> GVALGATRVIYPAGQKQEQLAVTNNDENSTYLIQSWVENADGVKDGRFIVTPPLFAMKGKKENTLRILDATNNQLPQDRESLFWMNVKAIPSMDKSKLTENTLQLAIISRIKLYYRPAKLALPPDQAAEKLRFRRSANSLTLINPTPYYLTVTELNAGTRVLENALVPPMGESTVKLPSDAGSNITYRTINDYGALTPKMTGVMEHHHH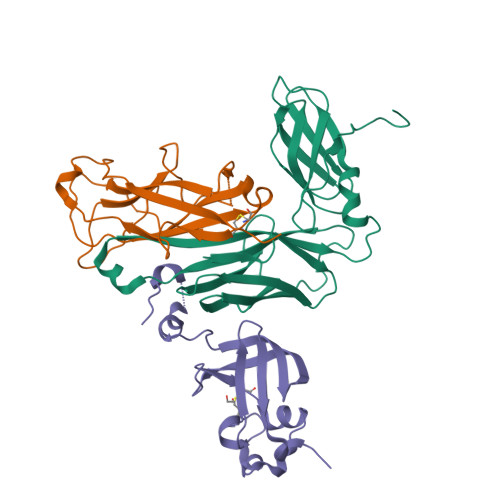HH;> DLYFNPRFLADDPQAVADLSRFENGQELPPGTYRVDIYLNNGYMATRDVTFNTGDSEQGIVPCLTRAQLASMGLNTASVAGMNLLADDACVPLTTMVQDATAHLDVGQQRLNLTIPQAFMSNRAR;> AETCRIEAGDKQMTVNMGQISSNRFHAVGEDSAPVPFVIHLRECSTVVSERVGVAFHGVADGKNPDVLSVGEGPGIATNIGVALFDDEGNLVPINRPPANWKRLYSGSTSLHFIAKYRATGRRVTGGIANAQAWFSLTYQ>[41x]MRINHNIAALNTLNRLSSNNSASQKNMEKLSSGLRINRAGDDAA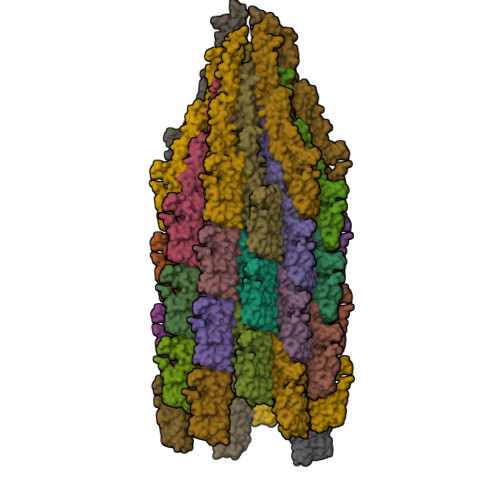GLAISEKMRGQIRGLEMASKNSQDGISLIQTAEGALTETHAILQRVRELVVQAGNTGTQDKATDLQSIQDEISALTDEIDGISNRTEFNGKKLLDGTYKVDTATPANQKNLVFQIGANATQQISVNIEDMGADALGIKEADGSIAALHSVNDLDVTKFADNAADCADIGFDAQLKVVDEAIYQVSSQRAKLGAVQNRLEHTINNLSASGENLTAAESRIRDVDMAKEMSEFTKNNILSQASQAMLAQANQQPQNVLQLLR> MRGRTLTLLARDALNAGSSMTLGSKGMRPSPEAHRRRMPWTAAKEYVPGVVLNSKEKLVLDGTQLVEL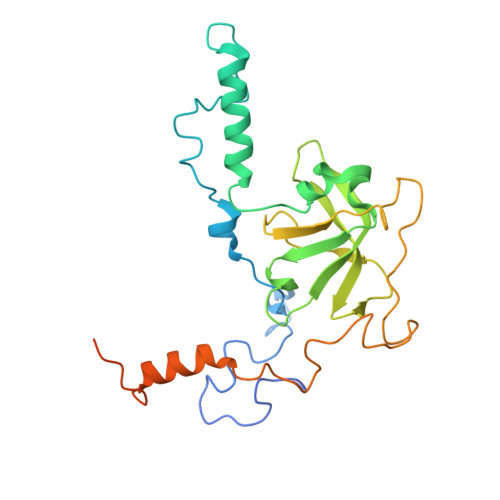DHIDRASQVDPLEVLKAAVATRAYNTSTGFNIFQLASQTRFHGRGQKFFREEWRQGTYEKYVTLAAIDFDREGSKGTAYGYITFHGESTTRPVEINYADTPGWQMEYDEAAAVPFDAAVPPPPSIGTEVPVDPSTYRLKAYPFYDAPNPPAFVERLLKDRGVLPDLPMDASAPAENAAAASADGALVDGSHHYESKGSV>[2x]GSMA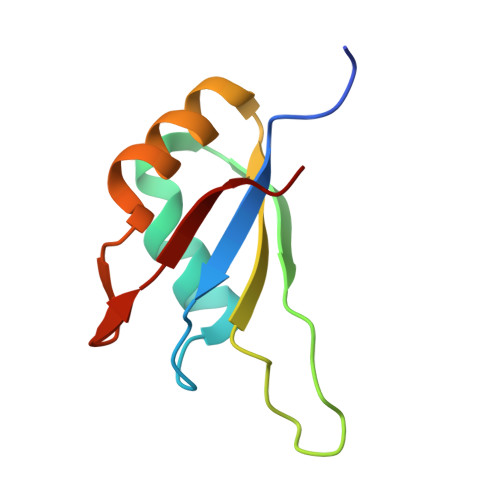TTKRVLYVGGLAEEVDDKVLHAAFIPFGDITDIQIPLDYETEKHRGFAFVEFELAEDAAAAIDNMNESELFGRTIRVNLAK> YQCHVCSAVLFSPLDLDAHVASHGLHGNMTLTSSDIQRHITEFISSWQNHPIVQVSADVENKKTAQLLHADTPRLVTWDAGLCTSFKIVPIVPAQVPQDVLAYTFFTSSYAIQSPFPEAAVSRIVVHTRWASNVDFDRDSSVIMAPPTENNIHLFKQLLNTETLSVRGANPLMFRANVLHMLLEFVLDNLYLNRHTGFSQDHTPFTEGANLRSLPGPDAEKWYSIMYPTRMGTPNVSKICNFVASCVRNRVGRFDRAQMMNGA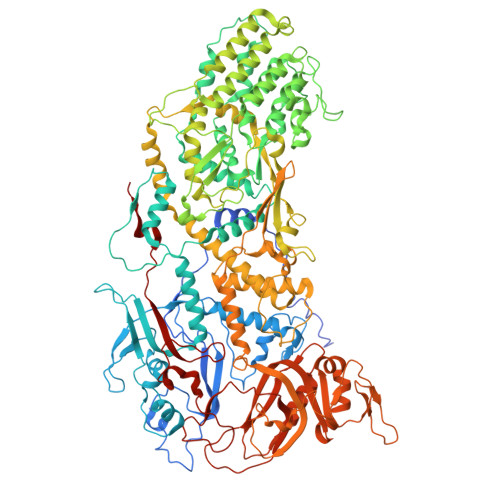MSEWVDVFETSDALTVSIRGRWMARLARMNINPTEIEWALTECAQGYVTVTSPYAPSVNRLMPYRISNAERQISQIIRIMNIGNNATVIQPVLQDISVLLQRISPLQIDPTIISNTMSTVSESTTQTLSPASSILGKLRPSNSDFSSFRVALAGWLYNGVVTTVIDDSSYPKDGGSVTSLENLWDFFILALALPLTTDPCAPVKAFMTLANMMVGFETIPMDNQIYTQSRRASAFSTPHTWPRCFMNIQLISPIDAPILRQWAEIIHRYWPNPSQIRYGAPNVFGSANLFTPPEVLLLPIDHQPANVTTPTLDFTNELTNWRARVCELMKNLVDNQRYQPGWTQSLVSSMRGTLDKLKLIKSMTPMYLQQLAPVELAVIAPMLPFPPFQVPYVRLDRDRVPTMVGVTRQSRDTITQPALSLSTTNTTVGVPLALDARAITVALLSGKYPPDLVTNVWYADAIYPMYADTEVFSNLQRDMITCEAVQTLVTLVAQISETQYPVDRYLDWIPSLRASAATAATFAEWVNTSMKTAFDLSDMLLEPLLSGDPRMTQLAIQYQQYNGRTFNIIPEMPGSVIADCVQLTAEVFNHEYNLFGIARGDIIIGRVQSTHLWSPLAPPPDLVFDRDTPGVHIFGRDCRISFGMNGAAPMIRDETGLMVPFEGNWIFPLALWQMNTRYFNQQFDAWIKTGELRIRIEMGAYPYMLHYYDPRQYANAWNLTSAWLEEITPTSIPSVPFMVPISSDHDISSAPAVQYIISTEYNDRSLFCTNSSSPQTIAGPDKHIPVERYNILTNPDAPPTQIQLPEVVDLYNVVTRYAYETPPITAVVMGVP> DSNENLLLVHCGPTLINSCISFGSESFDG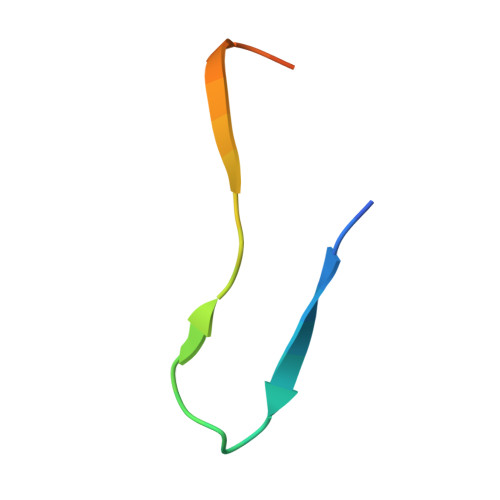H> NTKYNKEFLLYLA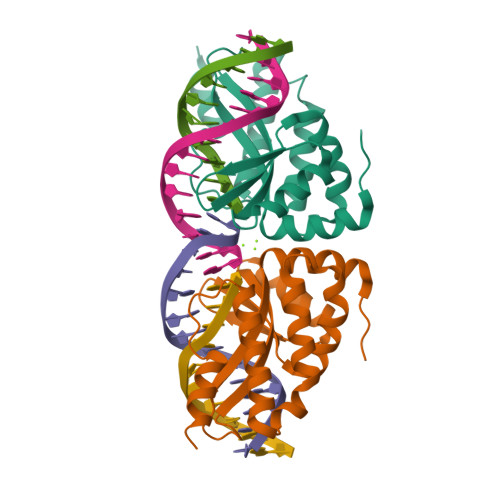GFVDSDGSIIAQIKPNQSVKFKHRLQLTFDVTQKTQRRWFLDKLVDEIGVGYVADSGSVSKYRLSEIKPLHNFLTQLQPFLKLKQKQANLVLKIIEQLPSAKESPDKFLEVCTWVDQIAALNDSKTRKTTSETVRAVLDSL;> NTKYNKEFLLYLAGFVDGDGSIIAQIKPNQSGKFKHKLSLTFKVTQKTQRRWFLDKLVDEIGVGYVYDSGSVSNYYLSEIKPLHNFLTQLQPFLKLKQKQANLVLKIIEQLPSAKESPDKFLEVCTWVDQVAALNDSKTRKTTSETVRAVLDSL> MIRAVFFDFVGTLLSVEGEAKTHLKIMEEVLGDYPLNPKTLLDEYEKLTREAFSNYAGKPYRPIRDIEEEVMRKLAEKYGFKYPENFWEIHLRMHQRYGELYPEVV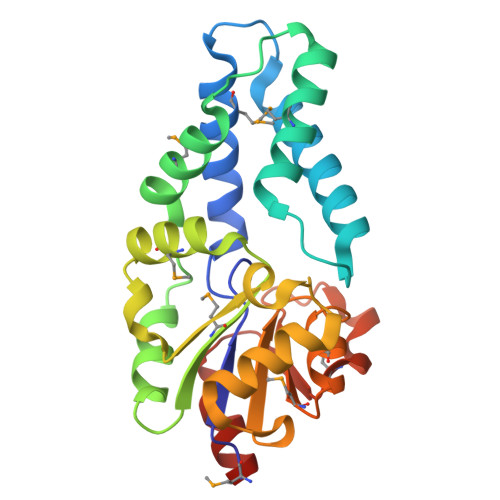EVLKSLKGKYHVGMITDSDTEYLMAHLDALGIKDLFDSITTSEEAGFFKPHPRIFELALKKAGVKGEEAVYVGDNPVKDCGGSKNLGMTSILLDRKGEKREFWDKCDFIVSDLREVIKIVDELNGQ> MPVRRGHVAPQNTFLDTIIRKFEGQSRKFIIANARVENCAVIYCNDGFCELCGYSRAEVMQRPCTCDFLHGPRTQRRAAAQIAQALLGAEERKVEIAFYRKDGSCFLCLVDVVPVKNEDGAVIMFILNFEVVMEKDMVGSGADVLPEYKLQAPRIHRWTILHYSPFKAVWDWLILLLVIYTAVFTPYSAAFLLKETEEGPPATECGYACQPLAVVDLIVDIMFIVDILINFRTTYVNANE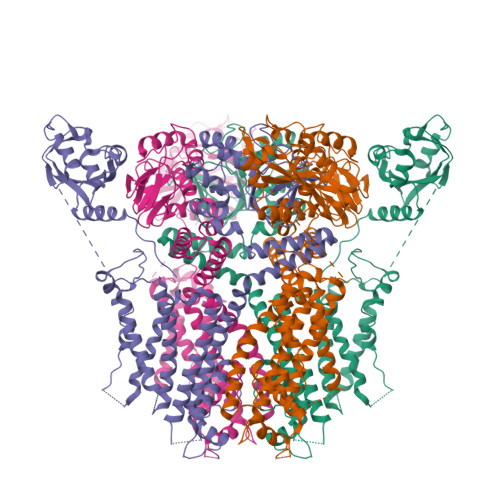EVVSHPGRIAVHYFKGWFLIDMVAAIPFDLLIFGSGSEELIGLLKTARLLRLVRVARKLDRYSEYGAAVLFLLMCTFALIAHWLACIWYAIGNMEQPHMDSRIGWLHNLGDQIGKPYNSSGLGGPSIKDKYVTALYFTFSSLTSVGFGNVAPNTNSEKIFSICVMLIGSLMYASIFGNVSAIIQRLYSGTARYHTQMLRVREFIRFHQIPNPLRQRLEEYFQHAWSYTNGIDMNAVLKGFPECLQADICLHLNRSLLQHCKPFRGATKGCLRALAMKFKTTHAPPGDTLVHAGDLLTALYFISRGSIEILRGDVVVAILGKNDIFGEPLNLYARPGKSNGDVRALTYCDLHKIHRDDLLEVLDMYPEFSDHFWSSLEITFNLRDTNMIPGGRQYQELPRCPAPTPSLLNIPLSSPGRRPRGDVESRLDALQRQLNRLETRLSADMATVLQLLQRQMTLVPPAYSAVTTPGPGPTSTSPLLPVSPLPTLTLDSLSQVSQFMACEELPPGAPELPQEGPTRRLSLPGQLGALTSQPLHRHGSDPGSEASNSLEVLFQ4,5,6,7-TETRABROMO-N,N-DIMETHYL-1H-BENZIMIDAZOL-2-AMINE 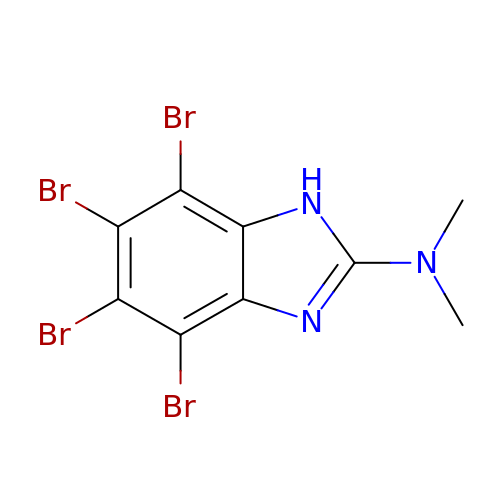| C9 H7 Br4 N3 | SLPJGDQJLTYWCI-UHFFFAOYSA-N>GSHMSRELKTVSADCKKEAIEKCAQWVVRDCRPFSAVSGSGFIDMIKFFIKVGAEYGEHVNVEELLPSPITLSRKVTSDAKEKKALISREIKSAVEKDGASATIDLWTDNYIKRNFLGVTLHYHENNELRDLILGLKSLDFERSTAENIYKKLKAIFSQFNVEDLSSIKFVTDRGANVVKSLANNIRINCSSHLLSNVLENSFEETPELNMPILACKNIVKYFKKANLQHRLRSSLKSECPTRWNSTYTMLRSILDNWESVIQILSEAGETQRIVHINKSIIQTMVNILDGFERIFKELQTCSSPSLCFVVPSILKVKEICSPDVGDVADIAKLKVNIIKNVRIIWEENLSIWHYTAFFFYPPALHMQQEKVAQIKE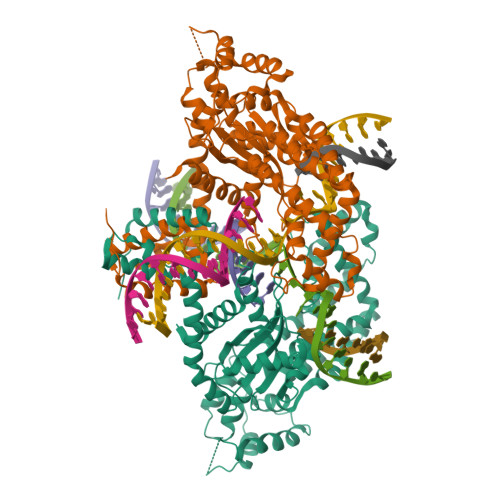FCLSKMEDLELINRMSSFNELSATQLNQSDSNSHNSIDLTSHSKPVSPSDEFEFYRKEIVILSEDFKVMEWWNLNSKKYPKLSKLALSLLSIPASSAASERTFSLAGNIITEKRNRIGQQTVDSLLFLNSFYKNFCKLDI[2x]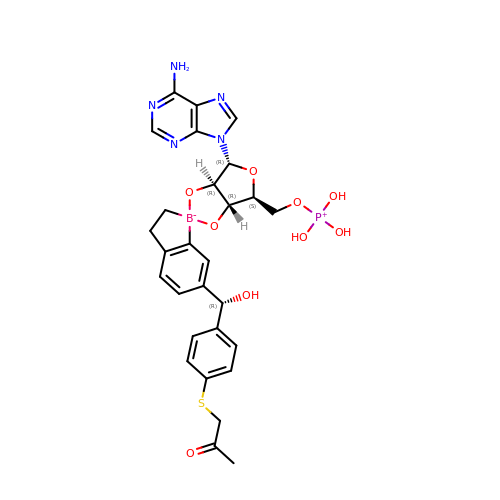[(1~{R},5~{R},6~{S},8~{R})-8-(6-aminopurin-9-yl)-4'-[(~{R})-oxidanyl-[4-(2-oxidanylidenepropylsulfanyl)phenyl]methyl]spiro[2,4,7-trioxa-3-boranuidabicyclo[3.3.0]octane-3,7'-7-boranuidabicyclo[4.3.0]nona-1(6),2,4-triene]-6-yl]methoxy-tris(oxidanyl)phosphanium | C28 H31 B N5 O9 P S | YYNKFKBRIAWSCO-QTPLPVLTSA-N>[2x]SDHSIEVTFRVKTQQVIIPEQNIRGNELPLRRWQMELLMLDATGKEVEPTILSKCIYHLHSSFKQPKRRLNSLPFFIKETGWGEFNLKIECFFIGNAGKFSIEHDLTFEDDAYAVDYTVDVPHEFSHLNSELSKYFDLP;> KQLASKAARKSAPSTGGVKY

Lysine benzoylation (Kbz) is a recently discovered post-translational modification associated with active transcription. Here, we systematically characterize writer, eraser, and reader proteins of histone Kbz in S. cerevisiae using proteomic, biochemical, and structural approaches. The Spt-Ada-Gcn5 acetyltransferase (SAGA) complex and NAD+-dependent histone deacetylase Hst2 could function as the writer and eraser of histone Kbz, respectively. In addition, we demonstrate that a subset of YEATS domains and bromodomains serve as Kbz readers, and structural analyses reveal how YEATS and bromodomains recognize Kbz marks.

To elucidate the molecular basis of Kbz recognition by the YEATS domains from Taf14YEATS and Sas5YEATS, we determined the crystal structures of the Taf14YEATS-H35-13K9bz and Sas5YEATS-H318-37K27bz complexes. In the 2.4 Å Sas5-H3K27bz structure, all H3 residues from K18 to K36 have well-defined electron density, including an extra tyrosine residue (Y37) at the C-terminus designed for concentration determination by UV spectrometry. The H3K27bz peptide binds to Sas5 in a partially similar configuration as the H3K27bz peptide in the hYEATS2-H3K27bz complex. Two H3K27bz peptides overlap at the target lysine (K27) and the flanking residues (A25-A31), but diverge at both the N- and C-termini. In the Sas5YEATS-H3K27bz structure, in addition to K27bz-mediated interactions, H3 A29 and P30 make extensive hydrophobic contacts with a hydrophobic groove composed of Sas5 L28, R31, W82, and F108. The downstream AP signatures are only observed in H3K14 and H3K27 peptides, explaining the relatively higher binding affinities of Sas5YEATS with H3K14 and H3K27 peptides than other peptides. Although H3K9bz and H3K27bz peptides show opposite orientations and their lysine side chains adopt different kinked configurations, their benzoyl groups are inserted into a conserved binding pocket sharing nearly identical interacting networks. The lysine side chains and the benzoyl groups are embraced by two arms: one arm is composed of a pentapeptide (residues 59–63 in Taf14 and residues 60-64 in Sas5), and the other arm is composed of a GWG motif that is the most conserved motif in all YEATS domains. A π-π-π stacking interaction composed of Taf14W81/Sas5W82, the benzene ring of Kbz, and Taf14F62/Sas5F63 dominantly determines the specific recognition of benzoylated lysine by YEATS domains. The Sas5 K64P mutant, which may generate a more closed binding pocket with increased hydrophobicity, substantially strengthened the interaction between Sas5YEATS and H3K27bz but only slightly increased the binding with H3K27ac.> GSKPVPIIA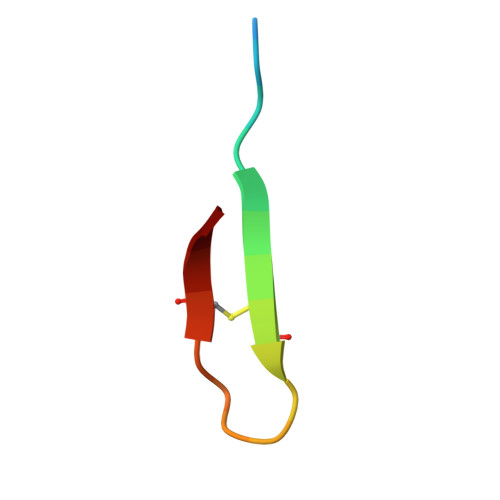CNRKTGKCRRI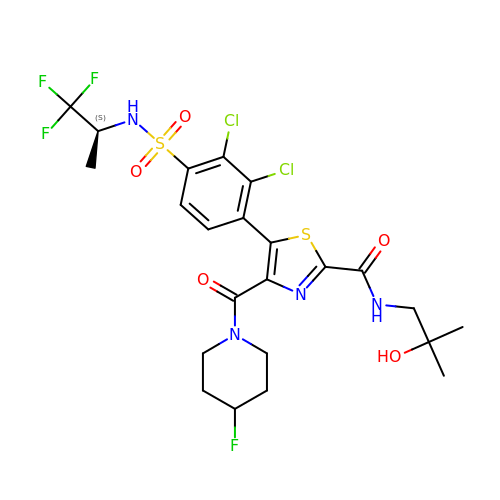5-(2,3-dichloro-4-{[(2S)-1,1,1-trifluoropropan-2-yl]sulfamoyl}phenyl)-4-(4-fluoropiperidine-1-carbonyl)-N-(2-hydroxy-2-methylpropyl)-1,3-thiazole-2-carboxamide | C23 H26 Cl2 F4 N4 O5 S2 | VZRCTKJCGGBKBW-NSHDSACASA-N> MEHVAFGSEDIENTLAKMDDGQLDGLAFGAIQLDGDGNILQYNAA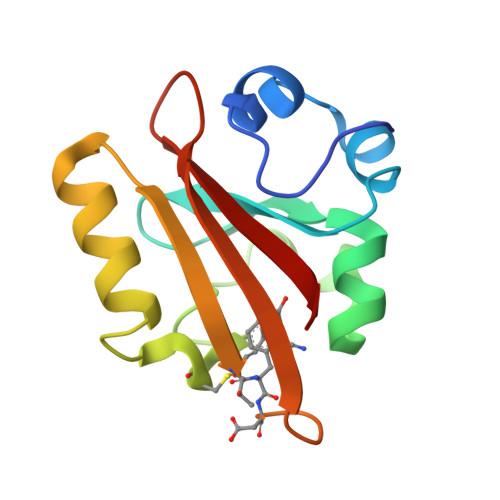EGDITGRDPKQVIGKNFFKDVAPCTDSPEFYGKFKEGVASGNLNTMFEYTXDYQDTPTKVKVHMKKALSGDSYWVFVKRV> MIERYSRPEMSAIWTDENRFQAWLEVEILACEAWAELGVIPKEDVKVMRENASFDINRILEIEKDTRHDVVAFTRAVSESLGEERKWVHYGLTSTDVVDTALSYLLKQANDILLKDLERFVDIIKEKAKEHKYTVMMGRTHGVHAEPTTFGLKLALWHEEMKRNLERFKQAKAGIEVGKISGAVGTYANIDPFVEQYVCEKLGLKAAPISTQTLQRDRHADYMATLALIATSIEKFAVEIRGLQKSETREVEEFFAKGQKGSSAMPHKRNPIGSENMTGMARVIRGYMMTAYENVPLWHERDISHSSAERIILPDATIALNYMLNRFSNIVKN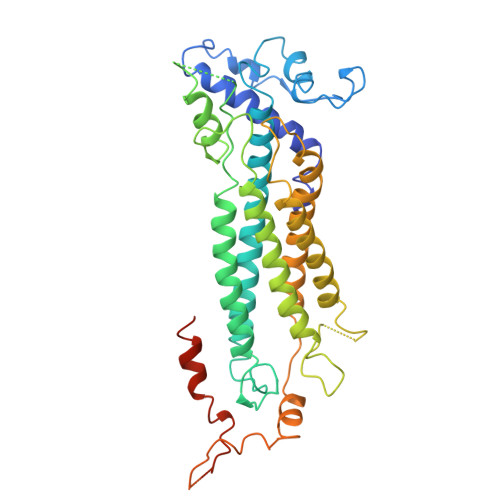LTVFPENMKRNMDRTLGLIYSQRVLLALIDTGLTREEAYDTVQPKAMEAWEKQVPFRELVEAEEKITSRLSPEKIADCFDYNYHLKNVDLIFERLGLA> MGEQVVKPTDERIIDPSTANTQLTGGVTYNTTSGGNKPLAGSPYGYETWIDTGGGVCSLTWYGADQGGGAAFKATWTNPHDFLGRLGYFWNENKPYSHYENIYCGFNYTRSGRKTAGDYSYIGIYGWSRNPSASNSNERLIEYYIVEDWFGNQWQADTSPMGINTTGGTVMGSFTCDGSSY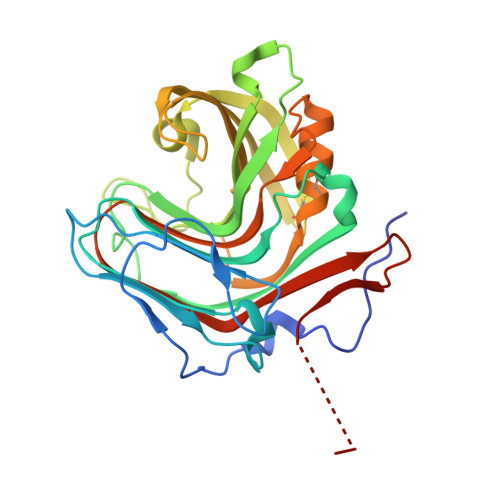QIIKNTRVNQPSIEGDKTFVQYFSIRQSPRKSGTISITCHFKKWEKLGMKLGDNMYECKFLIEAGAGEGFFDARLIQFYRADNEGNILQITPLEHHHHHH>[2x]GMRRGLVIVGHGSQLNHYREVMELHRKRIEESGAFDEVKIAFAARKRRPMPDEAIREMNCDIIYVVPLFISYGLHVTEDLPDLLGFPRGRGIKEGEFEGKKVVICEPIGEDYFVTYAILNS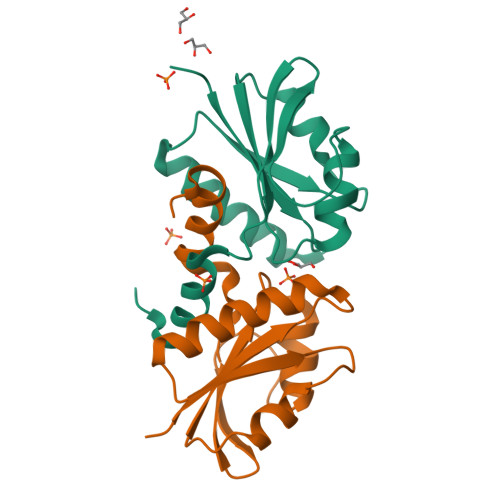VFRIGRDGKGEE6-methylpyridazin-3-ol | C5 H6 N2 O | 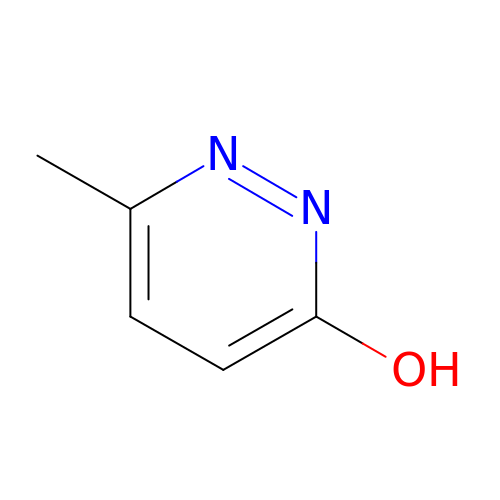QZWIXLPWMGHDDD-UHFFFAOYSA-N> MLARRSFLQAAAGSLVLGLARAQGPSFPEPKVVRSQGGLLSLKLSATPTPLAIAGQRATLLTYGGSFPGPTLRVRPRDTVRLTLENRLPEPTNLHWHGLPISPKVDDPFLEIPPGESWTYEFTVPKELAGTFWYHPHLHGRVAPQLFAGLLGALVVESSLDAIPELREAE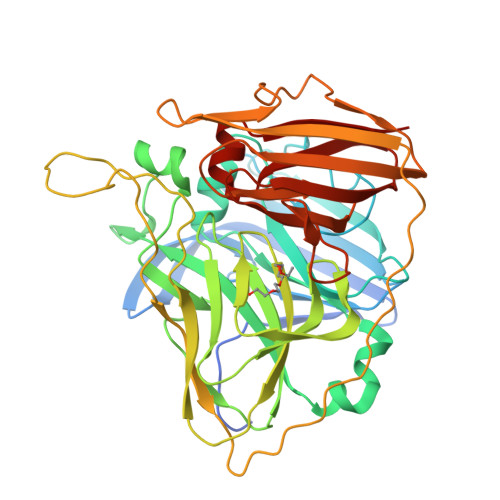EHLLVLKDLALQGGRPAPHTPMDWMNGKEGDLVLVNGALRPTLVAQKATLRLRLLNASNARYYRLALQDHPLYLIAADGGFLEEPLEVSELLLAPGERAEVLVRLRKEGRFLLQALPYDRGAMGMMDMGGMAHAMPQGPSRPETLLYLIAPKNPKPLPLPKALSPFPTLPAPVVTRRLVLTEDMMAARFFINGQVFDHRRVDLKGQAQTVEVWEVENQGDMDHPFHLHVHPFQVLSVGGRPFPYRAWKDVVNLKAGEVARLLVPLREKGRTVFHCHIVEHEDRGMMGVLEVG> SMAAFKPNSINYILGLDIGIASVGWAMVEIDEEENPIRLIDLGVRVFERAEVPKTGDSLAMARRLARSVRRLTRRRAHRLLRTRRLLKREGVLQAANFDENGLIKSLPNTPWQLRAAALDRKLTPLEWSAVLLHLIKHRGYLSQRKNEGETADKELGALLKGVAGNAHALQTGDFRTPAELALNKFEKESGHIRNQRSDYSHTFSRKDLQAELILLFEKQKEFGNPHVSGGLKEGIETLLMTQRPALSGDAVQKMLGHCTFEPAEPKAAKNTYTAERFIWLTKLNNLRILEQGSERPLTDTERATLMDEPYRKSKLTYAQARKLLGLEDTAFFKGLRYGKDNAEASTLMEMKAYHAISRALEKEGLKDKK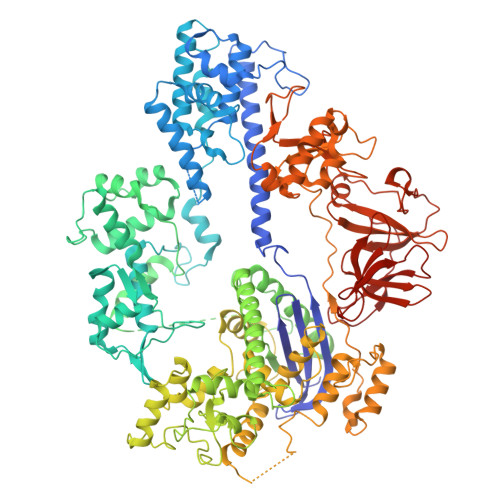SPLNLSPELQDEIGTAFSLFKTDEDITGRLKDRIQPEILEALLKHISFDKFVQISLKALRRIVPLMEQGKRYDEACAEIYGDHYGKKNTEEKIYLPPIPADEIRNPVVLRALSQARKVINGVVRRYGSPARIHIETAREVGKSFKDRKEIEKRQEENRKDREKAAAKFREYFPNFVGEPKSKDILKLRLYEQQHGKCLYSGKEINLGRLNEKGYVEIDHALPFSRTWDDSFNNKVLVLGSENQNKGNQTPYEYFNGKDNSREWQEFKARVETSRFPRSKKQRILLQKFDEDGFKERNLNDTRYVNRFLCQFVADRMRLTGKGKKRVFASNGQITNLLRGFWGLRKVRAENDRHHALDAVVVACSTVAMQQKITRFVRYKEMNAFDGKTIDKETGEVLHQKTHFPQPWEFFAQEVMIRVFGKPDGKPEFEEADTLEKLRTLLAEKLSSRPEAVHEYVTPLFVSRAPNRKMSGQGHMETVKSAKRLDEGVSVLRVPLTQLKLKDLEKMVNREREPKLYEALKARLEAHKDDPAKAFAEPFYKYDKAGNRTQQVKAVRVEQVQKTGVWVRNHNGIADNATMVRVDVFEKGDKYYLVPIYSWQVAKGILPDRAVVQGKDEEDWQLIDDSFNFKFSLHPNDLVEVITKKARMFGYFASCHRGTGNINIRIHDLDHKIGKNGILEGIGVKTALSFQKYQIDELGKEIRPCRLKKRPPVR>FQSMSRIALVTRLSPEAEAHWAGHLARALPGERIDGFRELSPAERAEVDIAIVANPDPADLAELPNLVWIHSLWAGVERLVAELGHLARPIVRLVDPELARTMAEAALAWTYYLFRDMPAYAAQQRARVWKGLPYKRPERTTVGVLGLGELGAAAALRLRDAGF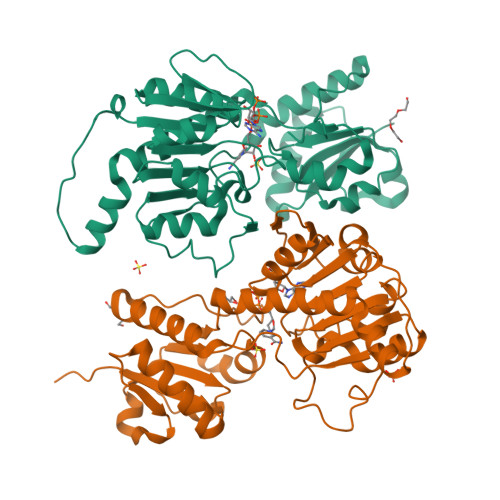DVHGWSRSPKEIAGVTCHAGEETLERMLGQVEILVCLLPLTGETRGLLDARRLACLPEGAQIVNFARGPILDSAALIEALDSGRIGHAVLDVFEVEPLPEASPFWGHPKVTVLPHISAATDPETASAIVGAHVADYRATGRIPPSVDLTRGY[2x]>MKHLISMKDIGKEEILEILDEARKMEELLNTKRPLKLLEGKILATVFYEPSTRTRLSFETAMKRLGGEVITMTDLKSSSVAKGESLIDTIRVISGYADIIVLRHPSEGAARLASEYSQVPIINAGDGSNQHPTQTLLDLYTIMREIGRIDGIKIAFVGDLKYGRTVHSLVYALSLFENVEMYFVSPKELRLPKDIIEDLKAKNIKFYEKESLDDLDDDIDVLYVTRIQKERFPDPNEYEKVKGSYKIKREYVEGKKFIIMHPLPRVDEID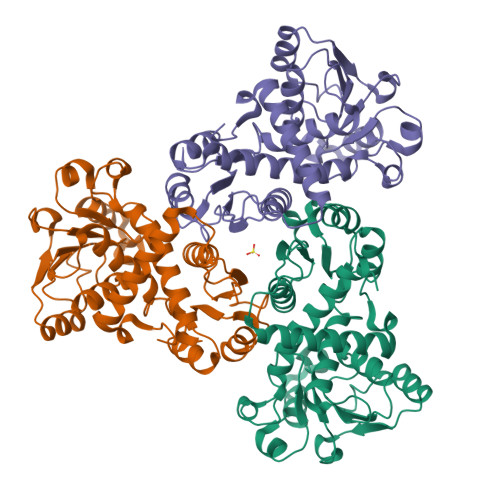YDVDDLPQAKYFKQSFYGIPVRMAILKKLIEDNEGE[12x]>[2x]MVESIFDALAHGRPLHHGYWAGGYREDAGATPWSDAADQLTDLFIDKAALRPGAHLFDLGCGNGQPVVRAACASGVRVTGITVNAQHLAAATRLANETGLAGSLEFDLVDGAQLPYPDGFFQAAWAMQSVVQIVDQAAAIREVHRILEPGGRFVLGDIITRVRLPEEYAAVWTGTTAHTLNSFTALVSEAGFEILEVTDLTAQTRCMVSWYVDELLRKLDELAGVEPAAVGTYQQRYLGDIAAKHGPGPA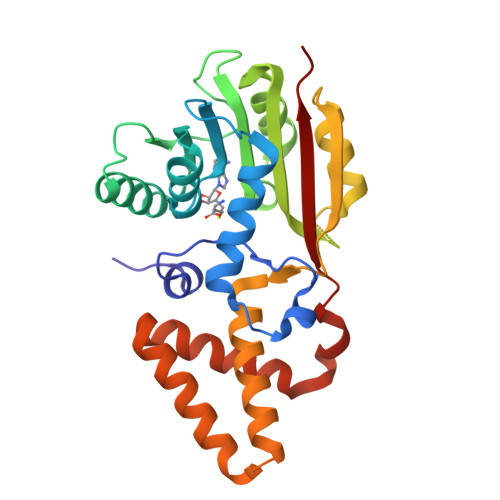QLIAAVAEYRKHPDYARNEESMGFMLLQARKKQS> GSWNEPYFDLTMPRNITSLVGKSAYLGCRVKHLGNKTVAWIRHRDLHILTVGTYTYTTDQRFQTSYHRDIDE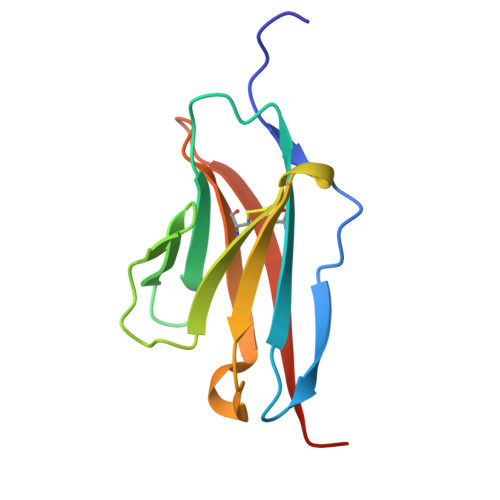WTLQIKWAQQRDAGVYECQISTQPVRSYSVNLNIVHHHHHH In nature, S‐adenosyl methionine (SAM)‐dependent methyltransferases efficiently catalyze this reaction with high stereoselectivity. This study presents the investigation and rational re‐design of a potential methyltransferase, termed SeMT, from the actinomycete Saccharopolyspora erythraea. A putative methyltransferase from Saccharopolyspora erythraea NRRL 2338, henceforth termed SeMT, was identified featuring 56% sequence identity with both StspM1 and SgMT. While its three‐dimensional structure elucidated via X‐ray crystallography confirmed extensive structural similarity to cyclic dipeptide‐processing methyltransferases such as SgMT, its putative catalytic center is clearly divergent. Accordingly, wild‐type SeMT displayed minimal activity with diketopiperazine (DKP) substrates, triggering an extensive mutagenesis effort aimed at iteratively enhancing this methyltransferase function.

Crystals of SeMT belong to orthorhombic space group C2221 and contain two copies of the protomer per asymmetric unit. As expected from the amino acid sequence similarity, SeMT features the same overall architecture as found for indole C3‐methyltransferases SgMT (Haase et al. 2025) and PsmD (Amariei et al. 2022), with the putative catalytic cavity located at the interface of a Rossmann‐type α/β domain and an all‐β cap domain. The two chains in the asymmetric unit are highly similar, featuring root‐mean‐square (RMS) distances of 0.55 Å both for 264 matching Cα atoms and for 1060 main‐chain atoms (least‐squares alignment using COOT (Emsley et al. 2010), using the prevalent conformer for residues with alternative conformations). In particular, the demethylated cofactor SAH (included in the sample for crystallization) is found embraced by a binding pocket that is virtually identical to the one found in those enzymes; this includes R82 and C60 essentially sandwiching the planar adenine ring, D81, which is hydrogen‐bonded to both hydroxyls of the ribose moiety, as well as E58 and R35 forming salt bridges with the homocysteine ammonium and carboxylate groups, respectively. Finally, the characteristic tyrosine side chains covering the cofactor (Y12, Y19, Y126) as well as the histidine‐acidic residue dyad thought to participate in catalysis (H218, E216) are retained. Indeed, while the catalytic cavity of SeMT resembles its counterpart in SgMT with respect to size (417 vs. 378 Å3, determined with the cofactor in place, average of chains A and B in either case) and overall character (hydrophobic patches dominated by aromatic side chains, interspersed with polar groups), residues at individual positions often differ notably in size and polarity. Preceding a regular and stable α‐helix (αA′), it features a more irregular terminal stretch we have termed the lid for its presumed role in controlling access to the active center during the catalytic cycle.

>[2x]MGHMTVDVPVSSDPYANLAASYDRLVDWVISEQEETPRERMGDYIESFWRDQPRPVHKVLEICCGTGLMLGDLQRRGYQVSGLDRSAAMLEQARNRLGTGVELVRAELPEIPLHAGFDAVISAANGLTYLPGTGFGETLAAVARLLPPGGTFVFDLYGHGFFERFYDSAEPRVLAVELEDVSYIWTFTAPPSRAHFDVVHSQFLRTPDAEAGTYTRTRELHRFHEHTHTSVRRLAAEAGFSSAEVHDNWTSRPSTPESMYDTWTLTRGVLEHHHHHH> EEPVPVPTEQTVFMYLPWSDNLTSNFYQNISDLESVVEKNILKDERIIIFMCTTATKATLFELAYENGKSVHKTLKNYTDPAYTTAEGITSILNDVQRYSPTKRYSMVIGCHGMGWIPVSNSKSRSGLRTKMH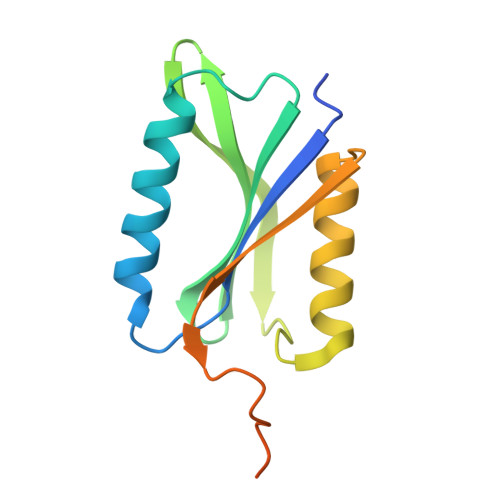WEYENVPMTR> MGHHHHHHENLYFQSNARKVQMGAKDATPVPCGRWAKILEKDKRTQQMRMQRLKAKLQMPFQSGEFKALTRRLQVEPRLLSKQMAGCLEDCTRQAPESPWEEQLARLLQEAPGKLSLDVEQAPSGQHSQAQLSGQQQRLLAFFKCCLLTDQLPLAHHLLVVHHGQRQKRKLLTLDMYNAVMLGWARQGAFKELVYVLFMVKDAGLTPDLLSYAAALQCMGRQDQDAGTIERCLEQMSQEGLKLQALFTAVLLSEEDRATVLKAVHKVKPTFSLPPQLPPPVNTSKLLRDVYAKDGRVSYPKLHLPLKTLQCLFEKQLHMELASRVCVVSVEKPTLPSKEVKHARKTLKTLRDQWEKALCRALRETKNRLEREVYEGRFSLYPFLCLLDEREVVRMLLQVLQALPAQGESFTTLARELSARTFSRHVVQRQRVSGQVQALQNHYRKYLCLLASDAEVPEPCLPRQYWEALGAPEALREQPWPLPVQMELGKLLAEMLVQATQMPCSLDKPHRSSRLVPVLYHVYSFRNVQQIGILKPHPAYVQLLEKAAEPTLTFEAVDVPMLCPPLPWTSPHSGAFLLSPTKLMRTVEGATQHQELLETCPPTALHGALDALTQLGNCAWRVNGRVLDLVLQLFQAKGCPQLGVPAPPSEAPQPPEAHLPHSAAPARKAELRRELAHCQKVAREMHSLRAEALYRLSLAQHLRDRVFWLPHNMDFRGRTYPCPPHFNHLGSDVARALLEFAQGRPLGPHGLDWLKIHLVNLTGLKKREPLRKRLAFAEEVMDDILDSADQPLTGRKWWMGAEEPWQTLACCMEVANAVRASDPAAYVSHLPVHQDGSCNGLQHYAALGRDSVGAASVNLEPSDVPQDVYSGVAAQVEVFRRQDAQRGMRVAQVLEGFITRKVVKQTVMTVVYGVTRYGGRLQIEKRLRELSDFPQEFVWEASHYLVRQVFKSLQEMFSGTRAIQHWLTESARLISHMGSVVEWVTPLGVPVIQPYRLDSKVKQIGGGIQSITYTHNGDISRKPNTRKQKNGFPPNFIHSLDSSHMMLTALHCYRKGLTFVSVHDCYWTHAADVSVMNQVCREQFVRLHSEPILQDLSRFLVKRFCSEPQKILEASQ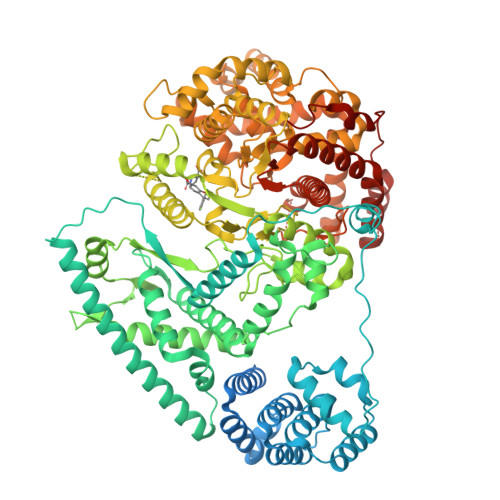LKETLQAVPKPGAFDLEQVKRSTYFFS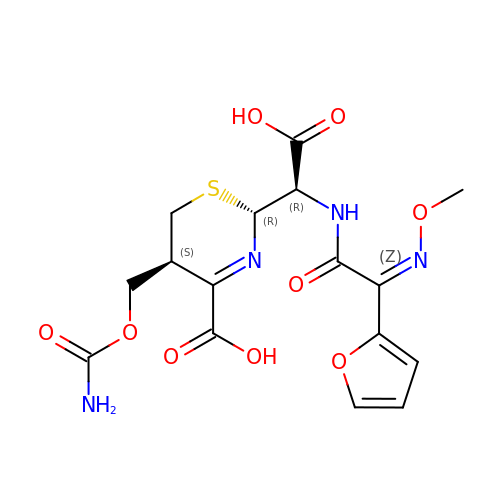(2R,5S)-5-[(carbamoyloxy)methyl]-2-[(R)-carboxy{[(2Z)-2-(furan-2-yl)-2-(methoxyimino)acetyl]amino}methyl]-5,6-dihydro-2H-1,3-thiazine-4-carboxylic acid | C16 H18 N4 O9 S | AYUIRPIPSPPXAA-NEHUYCMOSA-N>MGSDKIHHHHHHMIHFSINKNLFLQALNTTKRAISSKNAIPILSTVKIDVTNEGI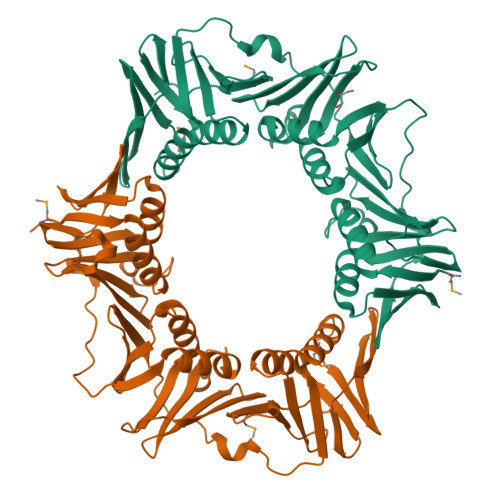TLIGSNGQISIENFISQKNEDAGLLITSLGSILLEASFFINVVSSLPDVTLDFKEIEQNQIVLTSGKSEITLKGKDSEQYPRIQEISASTPLILETKLLKKIINETAFAASTQESRPILTGVHFVLSQHKELKTVATDSHRLSQKKLTLEKNSDDFDVVIPSRSLREFSAVFTDDIETVEIFFANNQILFRSENISFYTRLLEGNYPDTDRLIPTDFNTTITFNVVNLRQSMERARLLSSATQNGTVKLEIKDGVVSAHVHSPEVGKVNEEIDTDQVTGEDLTISFNPTYLIDSLKALNSEKVTISFISAVRPFTLVPADTDEDFMQLITPVRTN[4x]>[2x]MTQFNITWEEQLQALSKLDGLHHPHKLEDISVHWVFNPVDISVFVTCATMSSHNTHYTFKPQSSPDDAMVREYVLSRIIADNLKYVDNLYLAAGAVICGNDEYISDGNVVGIHIADGVGGNKLILPVIEFMPGVHVDDISDKLIKSSSYQGIF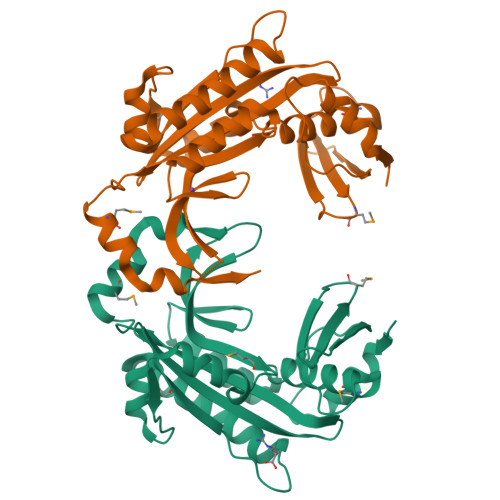KTDNLEEFEFLVDKKNANNVKELILAYTDYFANKLAFKDPAEPAVEMYQFIDRTEVYFSFEGCHPDVEEVLFTIKIVRYNQPLNSTAMQVFLKNPLLSHIRTVVRQDLPAKFVGGVLFNFKGHHHHHH> MKH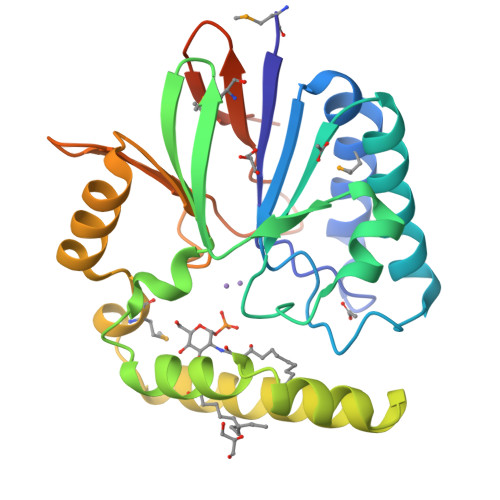SYFISDLHLSETQPELTALFVDFMQNLAPQAERLYILGDLFDFWIGDDEQSALIQQVKDLIKFVSDQGVQCYFQHGNRDFLIGERFSKETGAQLLPDYQLITLYDKKILLCHGDTLCIDDEAYQQFRRRVHQKWLQRLFLCLPLKVRVIIAEKIRAKSNQDKQAKSQEIMDVNQAFTAEKVQEFGVNLLIHGHTHREAIHQQEEFTRIVLGDWRKNYASILKMDESGEFGFIKDLEENLYFQSHHHHHHHHHH>[3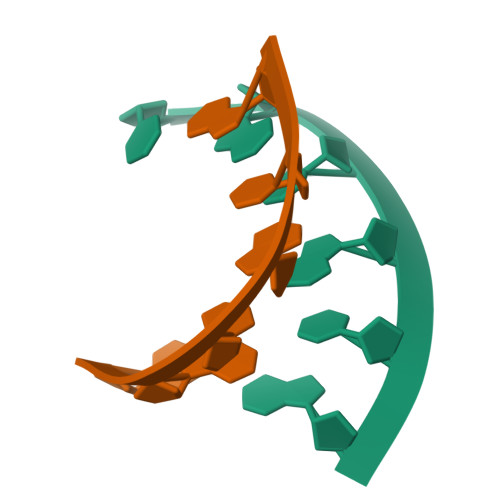x]CGCGXG Macrophage-expressed gene 1 (MPEG1, also termed Perforin-2) is one of the most ancient and highly conserved members of the membrane attack complex (MAC)/perforin-like (PF)/cholesterol-dependent cytolysin (MACPF/CDC) superfamily, with orthologous sequences identifiable throughout the metazoan. In contrast to other perforin-like proteins characterised to date, human MPEG1 is an integral type-1 transmembrane protein. The mature protein is comprised of three regions; an ectodomain located in the vesicular lumen, a transmembrane domain anchor that spans the vesicular membrane and, finally, a short cytosolic sequence. Each monomer of the 16-subunit ring possesses an N-terminal MACPF/CDC domain, a central multi-vesicular body of 12 kDa (MVB12)-associated β-prism (MABP) domain and a C-terminal region (termed the L-domain).

Indeed, our (ultimately unsuccessful) attempts to disrupt the interface between the double ring serendipitously led to our identifying the MPEG1 L425K mutation as yielding a greatly improved sample and an improvement in global resolution to 2.4 Å (workflow described in detail in the methods). This mutation resulted in two different MPEG1L425K assemblies, one of which involved domain swapping between the two head-to-head coordinated rings. In contrast to other MACPF/CDCs studied to date, the recombinant form of MPEG1 has pre-assembled into a soluble oligomer that exhibits the expected features of a prepore assembly. Within each subunit, both TMH-1 and -2 are folded as small helical bundles. A central feature of the assembly is a 64-stranded β-barrel that represents the top, preformed portion of the future pore. The majority of MACPF/CDC domain-mediated inter-subunit interactions are formed around the central lumen of the β-barrel. Around the outside of the assembly both the MABP domain and the L-domain also mediate extensive inter-subunit interactions. The L-domain forms substantial inter-subunit interactions in trans with an extraordinary elongated β-hairpin that extends from the MABP domain of the adjacent subunit (the MABP β-hairpin).

>KSGKPSGEMDEVGVQKCKNALKLPVLEVLPGGGWDNLRNVDMGRVMELTYSNCRTTEDGQYIIPDEIFTIPQKQSNLEMNSEILESWANYQSSTSYSINTELSLFSKVNGKFSTEFQRMKTLQVKDQAITTRVQVRNLVYTVKINPTLELSSGFRKELLDISDRLENNQTRMATYLAELLVLNYGTHVTTSVDAGAALIQEDHLRASFLQDSQSSRSAVTASAGLAFQNTVNFKFEENYTSQNVLTKSYLSNRTNSRVQSIGGVPFYPGITLQAWQQGITNHLVAIDRSGLPLHFFINPNMLPDLPGPLVKKVSKTVETAVKRYYTFNTYPGCTDLNSPNFNFQANTDDGSCEGKMTNFSFGGVYQECTQLSGNRDVLLCQKLEQKNPLTGDFSCPSGYSPVHLLSQIHEEGYNHLECHRKCTLKVFCKTVCEDVFQVAKAEFRAFWCVASSQVPENSGLLFGGLFSSKSINPMTNAQSCPAGYFPLRLFENLKVCVSQDYELGSRFAVPFGGFFSCTVGNPLVDPAISRDLGAPSLKKCPGGFSQHPALISDGCQVSYCVKSGLFTGGSLPPARLPPFTRPPLMSQAATNTVIVTNSENARSWIKDSQTHQWRLGEPIELRRAMNVIHGDGGGLSHHHHHH[16x]> GSHMGSPNSPLKDSLRPKLSEEQQHIIAILLDAHHKTYDPTYADFRDFRPPVRMDGSTGSVTLDLSPLSMLPHLADLVSYSIQKVIGFAKMIPGFRDLTSDDQIVLLKSSAIEVIMLRSNQS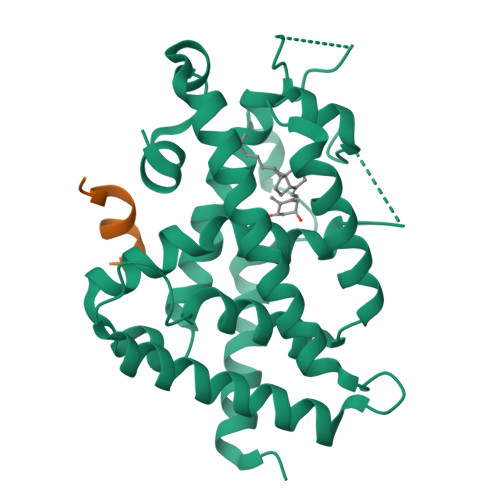FTMDDMSRDCGSQDYKYDVTDVSKAGHTLELIEPLIKFQVGLKKLNLHEEEHVLLMAICIVSPDRPGVQDAKLVEAIQDRLSNTLQTYIRCRHPPPGSHQLYAKMIQKLADLRSLNEEHSKQYRSLSFQPENSMKLTPLVLEVFGNEIS;> KNHPMLMNLLKDN> MSDEADEAYSVTEQLTMTGINRIRQKINAHGIP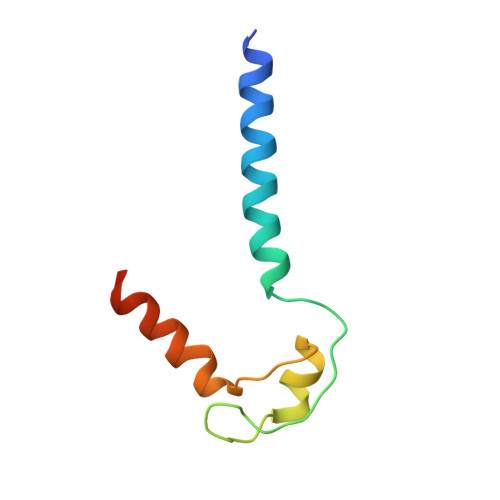VYLCEACGNPIPEARRKIFPGVTLCVECQAYQERQRKHYAHHHHHH> MSTSASGPEHE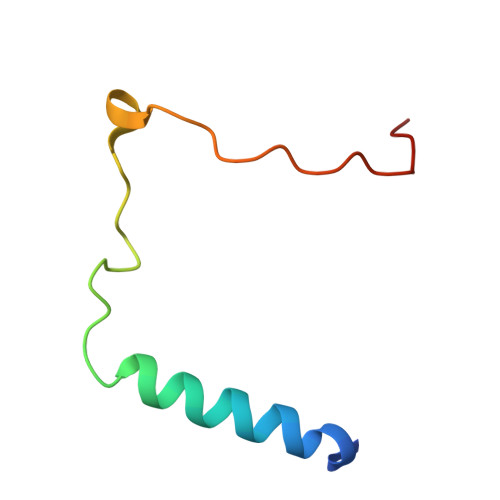FVSKFLTLATLTEPKLPKSYTKPLKDVTNLGVPLPTLKYKYKQ(2Z)-dodec-2-enoic acid | C12 H22 O2 | 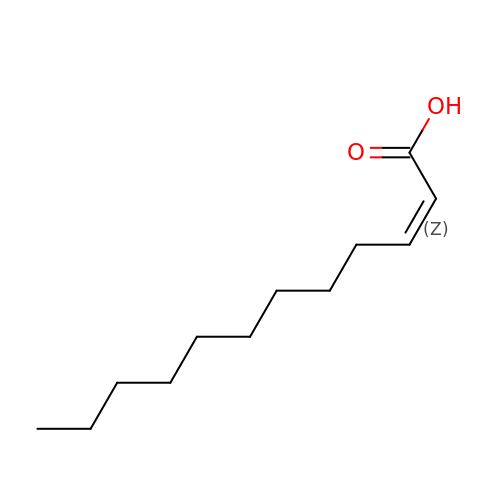PAWGRNGPMLVJQH-KHPPLWFESA-N> RRYRDERYPTQSPMPLTVACASPELASGKV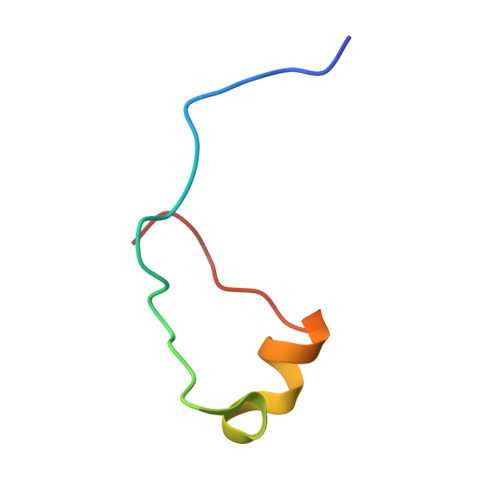WIRYPI> MNGIQVDINRLKKGEVSLGTSIMAVTF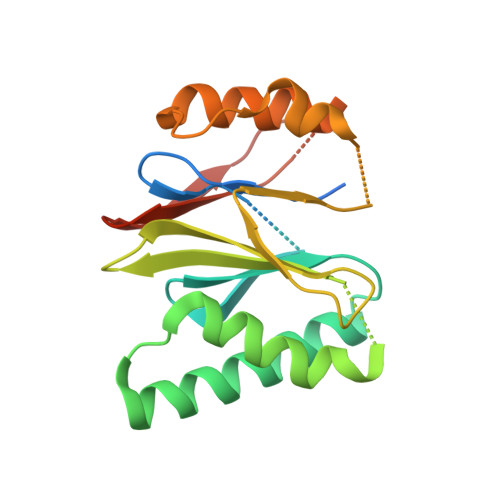KDGVILGADSRTTTGAYIANRVTDKLTRVHDKIWCCRSGSAADTQAIADIVQYHLELYTSQYGTPSTETAASVFKELCYENKDNLTAGIIVAGYDDKNKGEVYTIPLGGSVHKLPYAIAGSGSTFIYGYCDKNFRENMSKEETVDFIKHSLSQAIKWDGSSGGVIRMVVLTAAGVERLIFYPDEYEQL>MSLNNNDLVAKLWKLCDNLRDGGVSYQNYVNELASLLFLKMCKETGQEAEYLPEGYRWDDLKSRIGQEQLQFYRKMLVHLGEDDKKLVQAVFHNVSTTITEPKQITALVSNMDSLDWYNGAHGKSRDDFGDMYEGLLQKNANETKSGAGQYFTPRPLIKTIIHLLKPQPREVVQDPAAGTAGFLIEADRYVKSQTNDLDDLDGDTQDFQIHRAF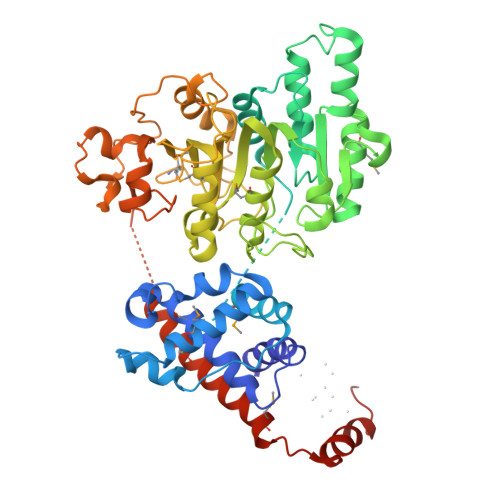IGLELVPGTRRLALMNCLLHDIEGNLDHGGAIRLGNTLGSDGENLPKAHIVATNPPFGSAAGTNITRTFVHPTSNKQLCFMQHIIETLHPGGRAAVVVPDNVLFEGGKGTDIRRDLMDKCHLHTILRLPTGIFYAQGVKTNVLFFTKGTVANPNQDKNCTDDVWVYDLRTNMPSFGKRTPFTDEHLQPFERVYGEDPHGLSPRTEGEWSFNAEETEVADSEENKNTDQHLATSRWRKFSREWIRTAKSDSLDISWLKDKDSIDADSLPEPDVLAAEAMGELVQALSELDALMRELGASDEADLQRQLLEEAFGGVKEEGGSHHHHHH[2x]>QNQYFTVQENYKERFYQIPKVFFTSENYKNLTNDMKIAYAILRDRLNLSIKNSWVDEDGNIYFVYSNEKLMEILNCKKEKLTKIKKGLENDGLLIQKRRGLNK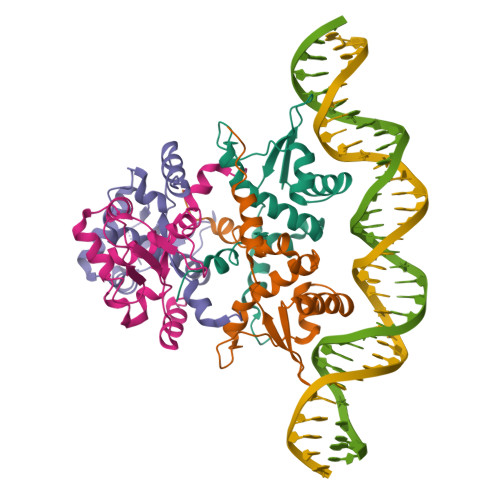PNILYLMKPIVTERDIYKIEKEENDVEPY[8x]> PISPIETVPVKLKPGMDGPKVKQWPLTEEKIKALVEICTEMEKEGKISKIGPENPYNTPVFAIKKKDSTKWRKLVDFRELNKRTQDFWEVQLGIPHPAGLKKKKSVTVLDVGDAYFSVPLDEDFRKYTAFTIPSINNETPGIRYQYNVLPQGWKGSPAIFQSSMTKILEPFRKQNPDIVIYQYMDDLYVGSDLEIGQHRTKIEELRQHLLRWGLTTPDKKHQKEPPFLWMGYELHPDKWTVQPIVLPEKDSWTVNDIQKLVGKLNWASQIYPGIKVRQLCKLLRGTKALTEVIPLTEEAEL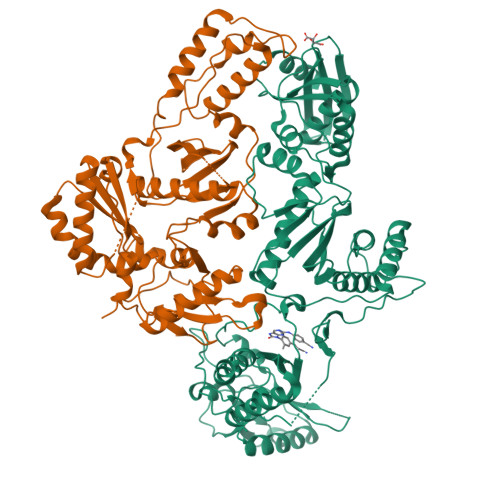ELAENREILKEPVHGVYYDPSKDLIAEIQKQGQGQWTYQIYQEPFKNLKTGKYARMRGAHTNDVKQLTEAVQKITTESIVIWGKTPKFKLPIQKETWETWWTEYWQATWIPEWEFVNTPPLVKLWYQLEKEPIVGAETFYVDGAANRETKLGKAGYVTNRGRQKVVTLTDTTNQKTELQAIYLALQDSGLEVNIVTDSQYALGIIQAQPDQSESELVNQIIEQLIKKEKVYLAWVPAHKGIGGNEQVDKLVSAGIRKVL;> PISPIETVPVKLKPGMDGPKVKQWPLTEEKIKALVEICTEMEKEGKISKIGPENPYNTPVFAIKKKDSTKWRKLVDFRELNKRTQDFWEVQLGIPHPAGLKKKKSVTVLDVGDAYFSVPLDEDFRKYTAFTIPSINNETPGIRYQYNVLPQGWKGSPAIFQSSMTKILEPFRKQNPDIVIYQYMDDLYVGSDLEIGQHRTKIEELRQHLLRWGLTTPDKKHQKEPPFLWMGYELHPDKWTVQPIVLPEKDSWTVNDIQKLVGKLNWASQIYPGIKVRQLCKLLRGTKALTEVIPLTEEAELELAENREILKEPVHGVYYDPSKDLIAEIQKQGQGQWTYQIYQEPFKNLKTGKYARMRGAHTNDVKQLTEAVQKITTESIVIWGKTPKFKLPIQKETWETWWTEYWQATWIPEWEFVNTPPLVKLWYQLEKEPIVGAETF>TCSTT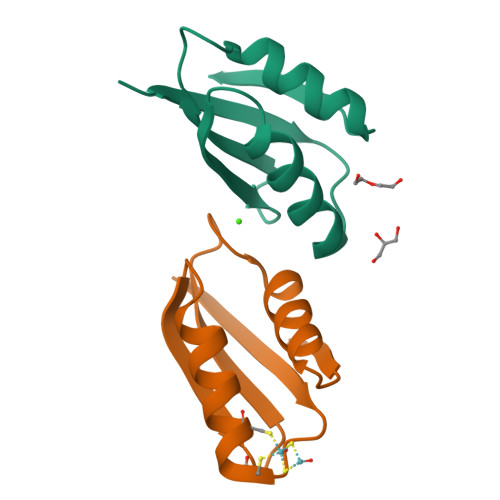LIAIAGMTCASCVHSIEGMISQLEGVQQISVSLAEGTATVLYNPAVISPEELRAAIEDMGFEASVVS[2x]> GGGUGGUGCG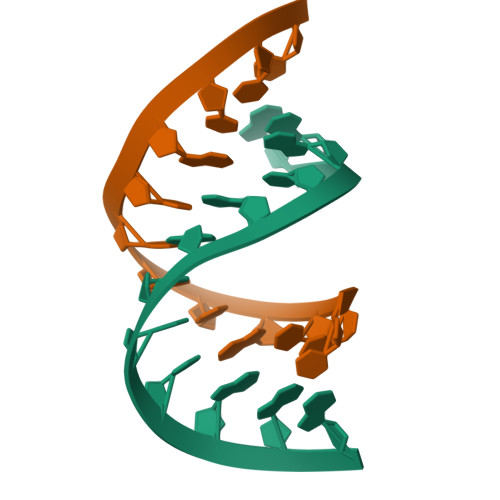GG;> CCUGCACUGCCC>[2x]GGVDREAMARCIEECLRCAQACTA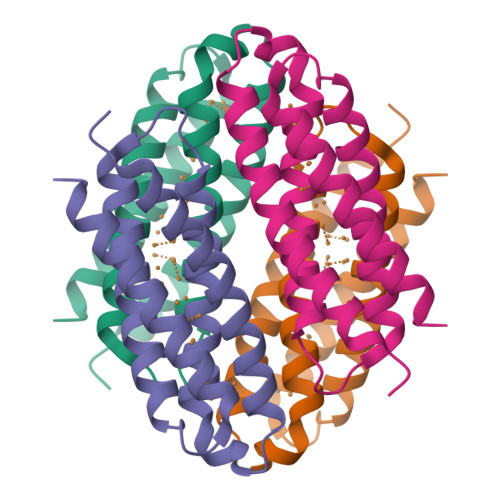CADACLSEPTVADLTKCIRTDMDCADVCTATAAVLSRHTGYDANVTRAVLQACATVCAACGDECARHAGMAEHCRVCAEACRSCEQACQELLAGLG Carboxylesterases are a family of enzymes that act on a variety of both exogenous (e.g. cocaine, heroin) and endogenous (e.g. acyl-CoA esters) substrates. They are defined by their ability to hydrolyze ester, amide, or thioester bonds to their corresponding alcohol, amine or thiol and free acid in a diverse range of chemically distinct compounds. Carboxylesterases comprise three distinct domains; a central domain containing the catalytic triad (S221, H467 and E354), a regulatory domain (RD) and an α/β domain. The active site occupies a 10-15Å deep hydrophobic pocket at the interface of the three domains with all three catalytic residues arranged such that a proton transfer chain can be established.

To provide a definitive insight into the importance of N-glycosylation on the structure and activity of human hCES1, the crystal structure of the enzyme with the mutation, N79Q, has been determined. The structure-function relationship of this aglycosylated hCES1 was explored alongside the wild type enzyme and a catalytically inactive mutant (S221A). Here, recombinant hCES1 enzymes were produced in HEK293 cells using either transient expression (hCES1 N79Q) or from stable cell lines (hCES1 and S221A). The yields of the aglycosylated hCES1 N79Q, glycosylated hCES1 and S221A enzymes were 39 mg/L, 64 mg/L and 68 mg/L respectively showing that N-glycosylation is not required for expression and secretion of the enzyme consistent with previous results. As expected, the mobility of the N79Q protein was not altered by PNGase treatment. Activity increased linearly with enzyme concentration and the specific activities for hCES1 and for hCES1 N79Q were 73 µmol min-1 μg-1, 98 µmol min-1 μg-1 respectively. Superposition of the monomeric structures showed no differences between the glycosylated and aglycosylated hCES1. A comparison of authentically glycosylated human hCES1 produced in HEK cells with an aglycosylated version of the enzyme shows that preventing glycosylation at N79 does not affect the synthesis, activity or structure of the enzyme.

> SPPVVDTVHGKVLGKFVSLEGFAQPVAIFLGIPFAKPPLGPLRFTPPQPAEPWSFVKQATSYPPMCTQDPKAGQLLSELFTNRKENIPLKLSEDCLYLNIYTPADLTKKNRLPVMVWIHGGGLMVGAASTYDGLALAAHENVVVVTIQYRLGIWGFFSTGDEHSRGNWGHLDQVAALRWVQDNIASFGGNPGSVTIFGESAGGESVSVLVLSPLAKNLFHRAISESGVALTSVLVKKGDVKPLAEQIAITAGCKTTTSAVMVHCLRQKTEEELLETTLKMKFLSLDLQGDPRESQPLLGTVIDGMLLLKTPEELQAERNFHTVPYMVGINKQEFGWLIPMLMSYPLSEGQLDQKTAMSLLWKSYPLVCIAKELIPEATEKYLGGTDDTVKKKDLFLDLIADVMFGVPSVIVARNHRDAGAPTYMYEFQYRPSFSSDMKPKTVIGDHGDELFSVFGAPFLKEGASEEEIRLSKMVMKFWANFARNGNPNGEGLPHWPEYNQKEGYLQIGANTQAAQKLKDKEVAFWTNLFAK>[2x]MYVCLCQGVTDNQIRDAIYEGC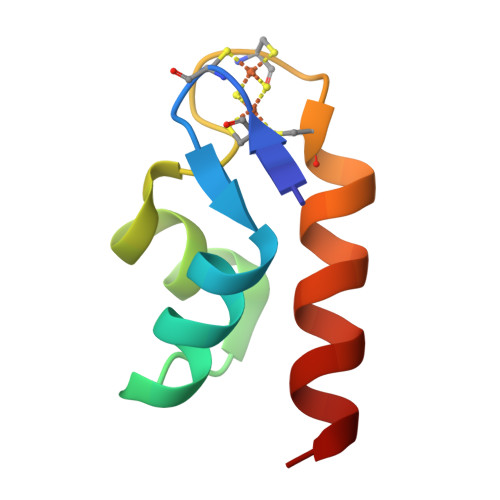CSYEEVREATGVGTQCGKCASLAYQVVRETLNDL>GAMGSMWKRSEQMKIKSGKCNMAAAMETEQLGVEIFETADCEENIESQDRPKLEPFYVERYSWSQLKKLLADTRKYHGYMMAKAPHDFMFVKRNDPDGPHSDRIYYLAMSGENRENTLFYSEIPKTINRAAVLMLSWKPLLDLFQATLDYGMYSREEELLRERKRIGTVGIASYDYHQGSGTFLFQAGSGIYHVKDGGPQGFTQQPLRPNLVETSCPNIRMDPKLCPADPDWIAFIHSNDIWISNIVTREERRLTYVHNELANMEEDARSAGVATFVLQEEFDRYSGYWWCPKAETTPSGGKILRILYEENDESEVEIIHVTSPMLETRRADSFRYPKTGTANPKVTFKMSEIMIDAEGRIIDVIDKELIQPFEILFEGVEYIARAGWTPE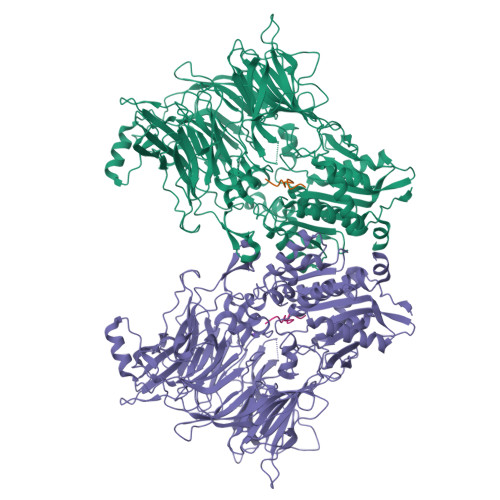GKYAWSILLDRSQTRLQIVLISPELFIPVEDDVMERQRLIESVPDSVTPLIIYEETTDIWINIHDIFHVFPQSHEEEIEFIFASECKTGFRHLYKITSILKESKYKRSSGGLPAPSDFKCPIKEEIAITSGEWEVLGRHGSNIQVDEVRRLVYFEGTKDSPLEHHLYVVSYVNPGEVTRLTDRGYSHSCCISQHCDFFISKYSNQKNPHCVSLYKLSSPEDDPTCKTKEFWATILDSAGPLPDYTPPEIFSFESTTGFTLYGMLYKPHDLQPGKKYPTVLFIYGGPQVQLVNNRFKGVKYFRLNTLASLGYVVVVIDNRGSCHRGLKFEGAFKYKMGQIEIDDQVEGLQYLASRYDFIDLDRVGIHGWSYGGYLSLMALMQRSDIFRVAIAGAPVTLWIFYDTGYTERYMGHPDQNEQGYYLGSVAMQAEKFPSEPNRLLLLHGFLDENVHFAHTSILLSFLVRAGKPYDLQIYPQERHSIRVPESGEHYELHLLHYLQENLGSRIAALKVI[3x];>SLRFLFEGQRIADNH[3x]> GAACGACACTGA;> CGGAGACTC;> TCACCG;> TCGAGTCTGTGTCGT

In this work, we exhaustively probe the ability of all 36 immobile HJ sequences to form DNA crystals in two different designed systems. Three separate self-assembling DNA crystal systems are described in this report: the “4 × 5” and “4 × 6” designs (collectively referred to as the 4 × N systems), and a third construct with a “scrambled” sequence variant of the 4 × 6 lattices. Self-assembly was mediated by three constituent oligonucleotides: (S1) containing four sequence repeats of either 5 or 6 bases; (S2) composed of 21 bases containing complementary regions to both (S1); and (S3) which forms the second junction crossover. The HJ serves as the fundamental component at the core of each unit, and the ultimate assembly of the full lattice is facilitated by the complementary 2-base sticky ends that tail each duplex.

To investigate this possibility, we designed “scrambled” sequences with targeted base substitutions, while maintaining GC content, along each “stem”. Contrary to the buffer preference observed with the native P32 crystals, the scrambled systems exhibited an exclusive preference towards low salt buffers, much like the native R3 crystals. Remarkably, only J1 and J2 retained the P32 symmetry, with all others yielding an R3 lattice. It is also noteworthy that J1 and J2 (P32), along with the R3 systems, also shared a preference for low salt conditions, unlike the original P32 crystals. There appeared to be only a marginal difference in the average cell lengths in the R3 scramble crystals (a = b = 113.04 c = 51.10) relative to the native 4 × 6 sequences: the a, b axis trended ~2 Å shorter and c ~1.3 Å longer, whereas in the J1 and J2 cases, the crystals were in good agreement with the original 4 × 6 motif. By contrast, the calculated angle for the P32 crystals was 58.05° (n = 2, σ = 1.39), compared with 54.60° (n = 16, σ = 1.44), a less accurate average due to a small sample size, so we posit that 54.60° more closely reflects the average observed angles in the 4 × 6 systems. However, in the majority of the crystal structures reported here, the cacodylate anion indeed fits best into the electron density map of our X-ray structures, due to the presence of sodium cacodylate in the crystallization solution.>[2x]GHMRKYSQRHIPVMVREVIEFLKPEDEKIILDCTVGEGGHSRAILEHCPGCRIIGIDVDSEVLRIAEEKLKEFSDRVSLFKVSYREADFLLKTLGI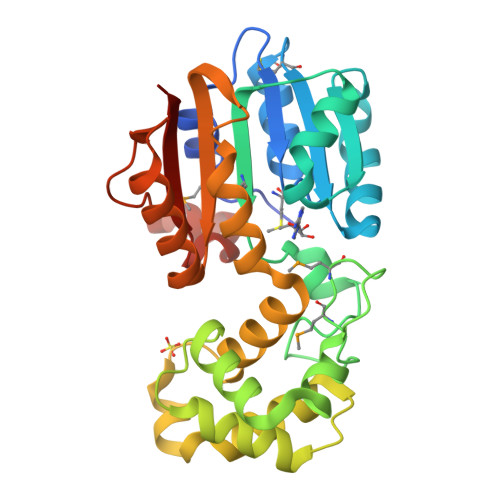EKVDGILMDLGVSTYQLKGENRGFTFEREEPLDMRMDLESEVTAQKVLNELPEEELARIIFEYGEEKRFARRIARKIVENRPLNTTLDLVKAVREALPSYEIRRRKRHFATKTFQAIRIYVNRELENLKEFLKKAEDLLNPGGRIVVISFHSLEDRIVKETFRNSKKLRILTEKPVRPSEEEIRENPRARSGRLRAAERIEEGGD> ETGDPKILKLSPETGPRQGGTRLTITGENLGLRFEDVRLGVHVGKVLCSP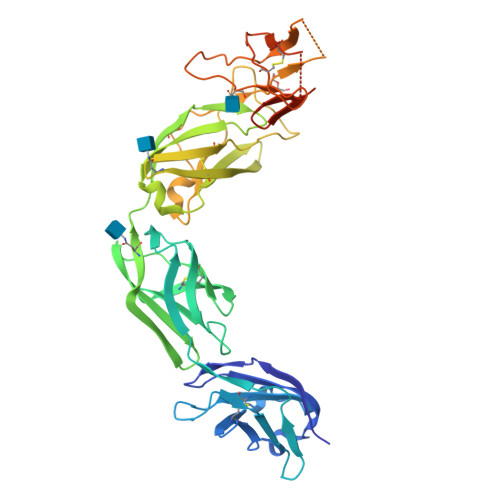VESEYISAEQIVCEIGDASTLRAHDALVEVCVRDCSLHYRALSPKRFTFVTPTFYRVSPSRGPLSGGTWIGIEGSHLNAGSDVAVSIGGRPCSFSWRNSREIRCLTPPGHTPGSAPIVININRAQLSNPEVKYNYTEDPTILRIDPEWSINSGGTLLTVTGTNLATVREPRIRAKYGGIERENSCMVYNDTTMVCRAPSIDNPKRSPPELGERPDEIGFIMDNVRTLLVLNSSSFLYYPDPVLEPLSPTGLLELKPSSPLILKGRNLLPPAPGNSRLNYTVLIGSTPCILTVSETQLLCEAPNLTGQHKVTVRAGGFEFSPGMLQVYSDSLLTLGTKHHHHHH> MGAIESRKLLASETPVGQFIPYSHHVTDTIISTKNAEYLSVWKIDGRSHQSASEADVFQWIRELNNTLRGISSANLSLWTHIVRRRVYEYPDAEFDNVFCRQLDEKYRESFTGYNLMVNDLYLTVVYRPVSDKVLSFFAKRERETPDQKKHRQESCIKALEDINRTLGQSFKRYGAELLSVYEKGGHAFSAPLEFLARLVNGEHIPMPICRDRFSDYMAVNRPMFSKWGEVGELRSLTGLRRFGMLEIREYDDATEPGQLNVLLESDYEFVLTHSFSVLSRPAAKEYLQRHQKNLIDARDVATDQIEEIDEALNQLISGHFVMGEHHCTLTVYGETVQQVRDNLAHASAAMLDVAVLPKPVDLALEAGYWAQLPANWQWRPRPAPITSLNFLSFSPFHNFMSGKPTGNPWGPAVTILKTVSGTPLYFNFHASKEEEDATDKRLLGN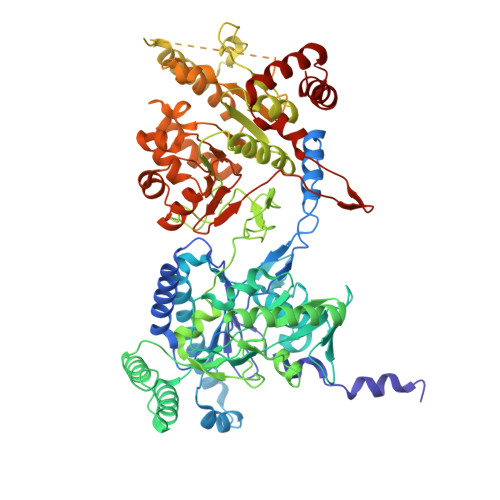TMLIGQSSSGKTVLLGFLLAQAQKFKPTIVAFDKDRGMEISIRAMGGRYLPLKTGEPSGFNPFQLPPTHANLIFLKQFVKKLAAAGGEVTHRDEEEIDQAITAMMSDSIDKSLRRLSLLLQFLPNPRSDDMDARPTVHARLVKWCEGGDYGWLFDNPTDALDLSTHQIYGFDITEFLDNPEARTPVMMYLLYRTESMIDGRRFMYVFDEFWKPLQDEYFEDLAKNKQKTIRKQNGIFVFATQEPSDALESNIAKTLIQQCATYIFLANPKADYEDYTQGFKLTDSEFELVRGLGEFSRRFLIKQGDQSALAEMNLGKFRTIVDGETVERDFDDELLVLSGTPDNAEIAESIIAEVGDDPAVWLPIFLDRVKAERSDV>[2x]MQKRAIYPGTFDPITNGHIDIVTRATQMFDHVILAIAASPSKKPMFTLEERVALAQQATAHLGNVEVVGFSDLMANFARNQHATVLIRGLRAVADFEYEMQLAHMNRHLMPELESVFLM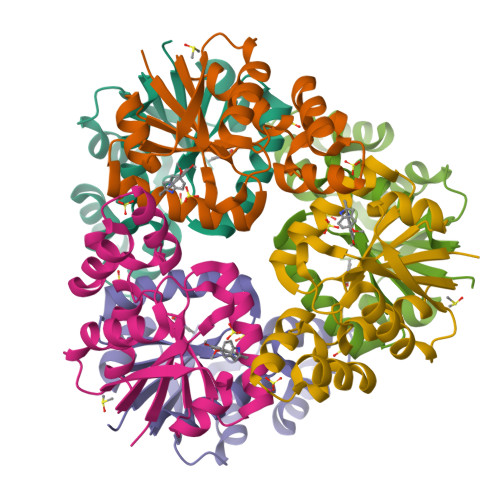PSKEWSFISSSLVKEVARHQGDVTHFLPENVHQALMAKLAVDHHHHHH>KAGVLKLPIESIHRDKDQPRTYFDEEKLKELSESIKAQGVLQPILVRKDGDGYRIIAGARRWRASQAAGLKEVPAIVRDVTEVQAFELALVENLQRADLNPIEEAEGYKRLVDEFKLTQEQVSVRVGKERSTVANALRLLALPTDVKGMVADGSLSMGHARALLGVPRLPELQNLAKQVADKKLSVRDTERLVQQ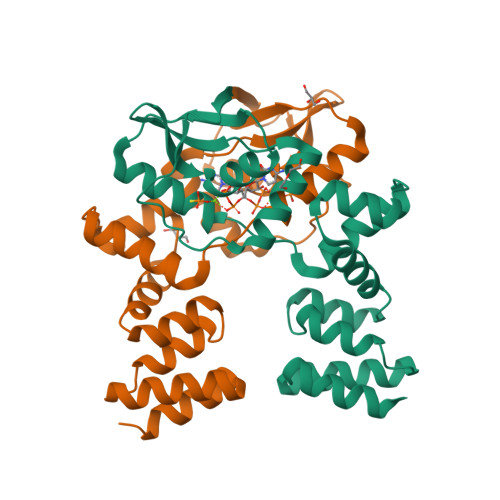SRSSGKKDAGKAAPKQS[2x]> ARARKGALVQCD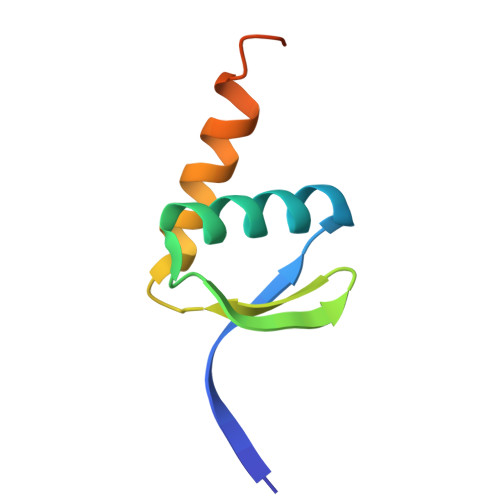PSIKALILQIDAKMSDIVLEELDDTHLLVNPSKVEFVKHELNRLLSKNIYNPMDEEENQ>MVKSRKISILLAVAMLVSIMIPTTAFAGPTKAPTKDGTSYKDLFLELYGKIKDPKNGYFSPDEGIPYHSIETLIVEAPDYGHVTTSEAFSYYVWLEAMYGNLTGNWSGVETAWKVMEDWIIPDSTEQPGMSSYNPNSPATYADEYEDPSYYPSELKFDTVRVGSDPVHNDLVSAYGPNMYLMHWLMDVDNWYGFGTGTRATFINTFQRGEQESTWETIPHPSIEEFKYGGPNGFLDLFTKDRSYAKQWRYTNAPDAEGRAIQAVYWANKWAKEQGKGSAVASVVSKAAKMGDFLRNDMFDKYFMKIGAQDKTPATGYDSAHYLMAWYTAWGGGIGASWAWKIGCSHAHFGYQNPFQGWVSATQSDFAPKSSNGKRDWTTSYKRQLEFYQWLQSAEGGIAGGATNSWNGRYEKYPAGTSTFYGMAYVPHPVYADPGSNQWFGFQAWSMQRVMEYYLETGDSSVKNLIKKWVDWVMSEIKLYDDGTFAIPSDLEWSGQPDTWTGTYTGNPNLHVRVTSYGTDLGVAGSLANALATYAAATERWEGKLDTKARDMAAELVNRAWYNFYCSEGKGVVTEEARADYKRFFEQEVYVPAGWSGTMPNGDKIQPGIK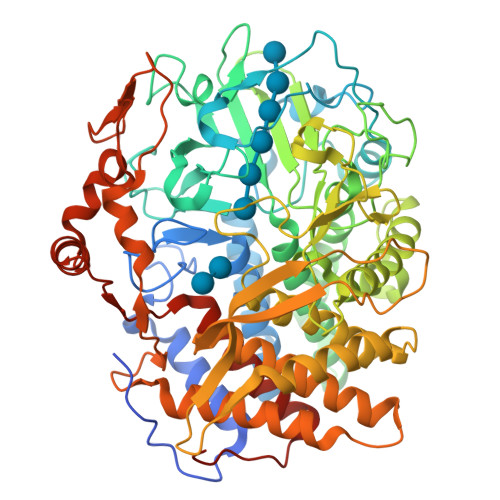FIDIRTKYRQDPYYDIVYQAYLRGEAPVLNYHRFWHEVDLAVAMGVLATYFPDMTYKVPGTPSTKLYG[6x]In Gram-negative bacteria, conjugation is mediated by a large transport apparatus—the conjugative type IV secretion system (T4SS)—produced by the donor cell and embedded in both its outer and inner membranes. The T4SS also elaborates a long extracellular filament—the conjugative pilus—that is essential for DNA transfer. Here we present a single-particle cryo-EM structure of a T4SS complex from the R388 plasmid that comprises all four sub-complexes: OMCC, stalk, arches and IMC. Three ATPases, VirB4 (also known as TrwK), VirB11 (also known as TrwD) and VirD4, power the system.

The arches (the composition and architecture of which were previously unknown) are composed of hexamers of homotrimeric units of VirB8peri, forming a 177 Å diameter ring around the stalk. The arches, comprising the VirB8 periplasmic domains (VirB8peri), also form a hexameric assembly with variable occupancy. Six VirB8peri homotrimeric units come together using the β1–β4 sheet on both sides. Near-atomic resolution was achieved for all except for the arches sub-complex.

>[3x]MSKKQPKPVKAEQLKSYYEESRGLERDLIGEFVKSRKTAWRVATASGLFGLLGMVCGIVGFSQPAPAPLVLRVDNATGAVDVVTTLREHESSYGEVVDTYWLNQYVLNREAYDYNTIQMNYDTTALLSAPAVQQDYYKLFDGSNARDRVLGNKARITVRVRSIQPNGRGQATVRFTTQQHNSNGTVEAPQHQIATIGYTYIGAPMRSSDRLLNPLGFQVTSYRADPEILNN2-[(2-cyano-3-fluoro-5-hydroxyphenyl)sulfanyl]ethanesulfonic acid | C9 H8 F N O4 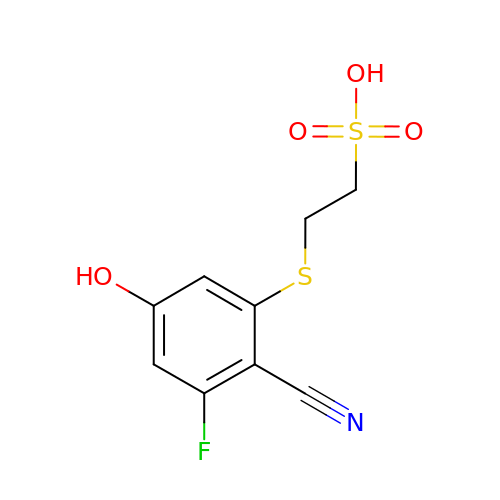S2 | ZFJOGPQOJAOGAK-UHFFFAOYSA-N>[4x]MPEVRAERYIPAPPERVYRLAKDLEGLKPYLKEVESLEVVAREGAR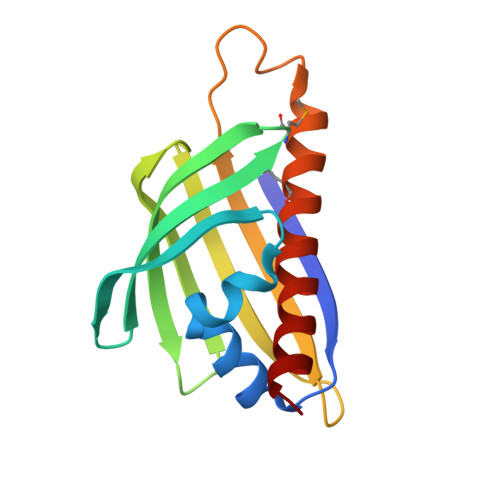TRSRWVAVAMGKKVRWLEEEEWDDENLRNRFFSPEGDFDRYEGTWVFLPEGEGTRVVLTLTYELTIPIFGGLLRKLVQKLMQENVESLLKGLEERVLAASS> PTE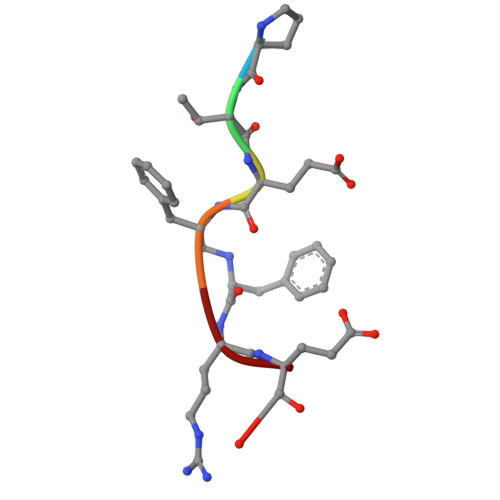XRE> MMDLVLEEDVTVPGTLSGCSGLVPSVPDDLDGINPNAGLGNGLLPNVSEETVSPTRARNMKDFENQITELKKENFNLKLRIYFLEERMQQEFHGPTEHIYKTNIELKVEVESLKRELQEREQLLIKASKAVESLAEAGGSEIQRVKEDARKKVQQVEDLLTKRILLLEKDVTAAQAELEKAFAGTETEKALRLRLESKLSEMKKMHEGDLAMALVLDEKDRLIEELKLSLKSKEALIQCLKEEKSQMACPDENVSSGELRGLCAAPREEKERETEAAQMEHQKERNSFEERIQALEEDLREKEREIATEKKNSLKRDKAIQGLTMALKSKEKKVEELNSEIEKLSAAFAKAREALQKAQTQEFQGSEDYETALSGKEALSAALRSQNLTKSTENHRLRRSIKKITQELSDLQQERERLEKDLEEAHREKSKGDCTIRDLRNEVEKLRNEVNEREKAMENRYKSLLSESNKKLHNQEQVIKHLTESTNQKDVLLQKFNEKDLEVIQQNCYLMAAEDL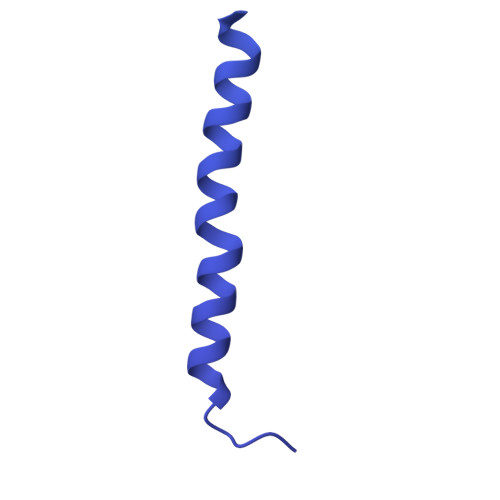ELRSEGLITEKCSSQQPPGSKTIFSKEKKQSSDYEELIQVLKKEQDIYTHLVKSLQESDSINNLQAELNKIFALRKQLEQDVLSYQNLRKTLEEQISEIRRREEESFSLYSDQTSYLSICLEENNRFQVEHFSQEELKKKVSDLIQLVKELYTDNQHLKKTIFDLSCMGFQGNGFPDRLASTEQTELLASKEDEDTIKIGEDDEINFLSDQHLQQSNEIMKDLSKGGCKNGYLRHTESKISDCDGAHAPGCLEEGAFINLLAPLFNEKATLLLESRPDLLKVVRELLLGQLFLTEQEVSGEHLDGKTEKTPKQKGELVHFVQTNSFSKPHDELKLSCEAQLVKAGEVPKVGLKDASVQTVATEGDLLRFKHEATREAWEEKPINTALSAEHRPENLHGVPGWQAALLSLPGITNREAKKSRLPILIKPSRSLGNMYRLPATQEVVTQLQSQILELQGELKEFKTCNKQLHQKLILAEAVMEGRPTPDKTLLNAQPPVGAAYQDSPGEQKGIKTTSSVWRDKEMDSDQQRSYEIDSEICPPDDLASLPSCKENPEDVLSPTSVATYLSSKSQPSAKVSVMGTDQSESINTSNETEYLKQKIHDLETELEGYQNFIFQLQKHSQCSEAIITVLCGTEGAQDGLSKPKNGSDGEEMTFSSLHQVRYVKHVKILGPLAPEMIDSRVLENLKQQLEEQEYKLQKEQNLNMQLFSEIHNLQNKFRDLSPPRYDSLVQSQARELSLQRQQIKDGHGICVISRQHMNTMIKAFEELLQASDVDYCVAEGFQEQLNQCAELLEKLEKLFLNGKSVGVEMNTQNELMERIEEDNLTYQHLLPESPEPSASHALSDYETSEKSFFSRDQKQDNETEKTSVMVNSFSQDLLMEHIQEIRTLRKRLEESIKTNEKLRKQLERQGSEFVQGSTSIFASGSELHSSLTSEIHFLRKQNQALNAMLIKGSRDKQKENDKLRESLSRKTVSLEHLQREYASVKEENERLQKEGSEKERHNQQLIQEVRCSGQELSRVQEEVKLRQQLLSQNDKLLQSLRVELKAYEKLDEEHRRLREASGEGWKGQDPFRDLHSLLMEIQALRLQLERSIETSSTLQSRLKEQLARGAEKAQEGALTLAVQAVSIPEVPLQPDKHDGDKYPMESDNSFDLFDSSQAVTPKSVSETPPLSGNDTDSLSCDSGSSATSTPCVSRLVTGHHLWASKNGRHVLGLIEDYEALLKQISQGQRLLAEMDIQTQEAPSSTSQELGTKGPHPAPLSKFVSSVSTAKLTLEEAYRRLKLLWRVSLPEDGQCPLHCEQIGEMKAEVTKLHKKLFEQEKKLQNTMKLLQLSKRQEKVIFDQLVVTHKILRKARGNLELRPGGAHPGTCSPSRPGS>GPHMAIHILTEKEDHATLHISFNDLIKIQLRTNPSTGYAWNIEYPTDTFSLSQDTIKAEPHPSGMVGFPSIREIQLKPLKVGTTTIKLGYSRPWEKGKEPLRSLTYSVVIR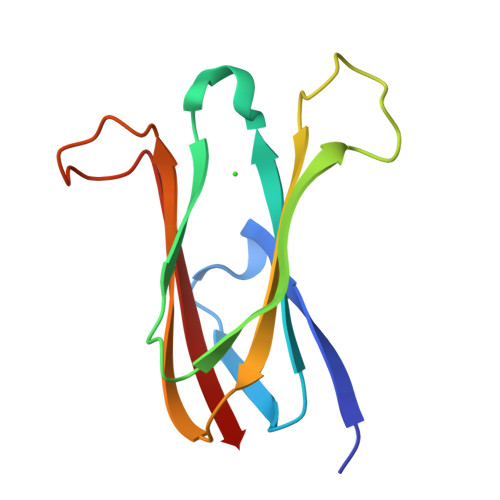[2x]In these experiments, bacterial proteins with different functions were investigated. Microcrystals of photoactive yellow protein (PYP), a blue-light photoreceptor from Halorhodospira halophila, were used to explore the capability of microsecond X-ray pulses. A nitrite-reducing enzyme, cytochrome c nitrite reductase (ccNiR) from Shewanella oneidensis, was exploited to investigate potential secondary radiation damage, caused by 90 µs pulses, at heme centers. Finally, a first TR-SSX experiment was performed on the photosensory core module (PCM) of a bacterial phytochrome from the nonphotosynthetic myxobacterium Stigmatella aurantiaca.

CcNiR is a decaheme enzyme that catalyzes the six-electron reduction of nitrite to ammonia. It is an important enzyme in the nitrogen cycle and is essential in agriculture for ammonia generation from nitrate fertilizers. CcNiR crystallized in space group P212121 with a dimer in the asymmetric unit. The PEG is situated far away from the opening of the channels that guide ions, electrons and water into the active heme coordination sites. Very weak, if any, tell-tale DED is detectable near any of the ten heme irons in ccNiR Fo − Fc difference maps.

>[2x]SDKTEPRNEVYKDKFKNQYNSWHDTAKSEELVDALEQDPNMVILWAGYAFAKDYKAPRGHMYAVTDVRNTLRTGAPKNAEDGPLPMACWSCKSPDVPRLIEEQGEDGYFKGKWAKGGPEVTNTIGCSDCHEKGSPKLRISRPYVDRALDAIGTPFSKASKQDKESMVCAQCHVEYYFEKKEDKKGFVKFPWDMGVTVDQMEVYYDGIEFSDWTHALSKTPMLKAQHPEYETWKMGIHGKNNVSCVDCHMPKVTSPEGKKFTDHKVGNPFDRFEETCATCHSQTKEFLVGVTNERKAKVKEMKLKAEEQLVKAHFEAAKAWELGATEAEMKPILTDIRHAQWRWDLAIASHGVAAHAPEEALRVLGTSVNKAADARVKLAQLLAKKGLTDPVAIPDISTKAKAQAVLGMDMEKMNAEKEAFKKDMLPKWDAEAKKREATY>[4x]MEDENILRNAVNLQVLKFHYPEIESIIDIASHVAVYQFDVGSQKWLKTSIEGTFFLVKDQRARVGYVILNRNSPENLYLFINHPSNVHLVDRYLIHRTENQHVVGLWMFDPNDMSRIFNIVKESLLR;>MS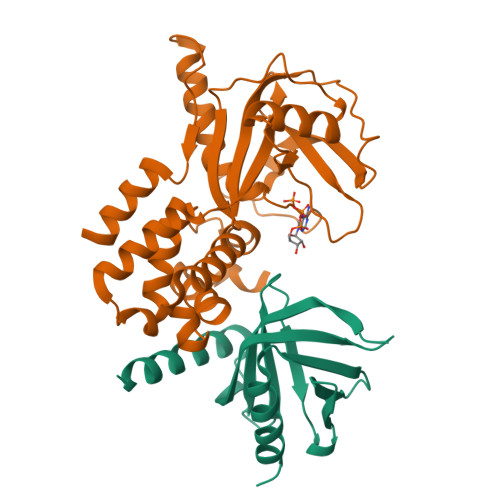FTNATFSQVLDDLSARFILNLPAEEQSSVERLCFQIEQAHWFYEDFIRAQNDQLPSLGLRVFSAKLFAHCPLLWKWSKVHEEAFDDFLRYKTRIPVRGAIMLDMSMQQCVLVKGWKASSGWGFPKGKIDKDESDVDCAIREVYEETGFDCSSRINPNEFIDMTIRGQNVRLYIIPGISLDTRFESRTRKEISKIEWHNLMDLPTFKKNKPQTMKNKFYMVIPFLAPLKKWIKKRNIANNTTKEKNISVDVDADASSQLLSLLKS[4x]> MISNNAPAKMVLNSIM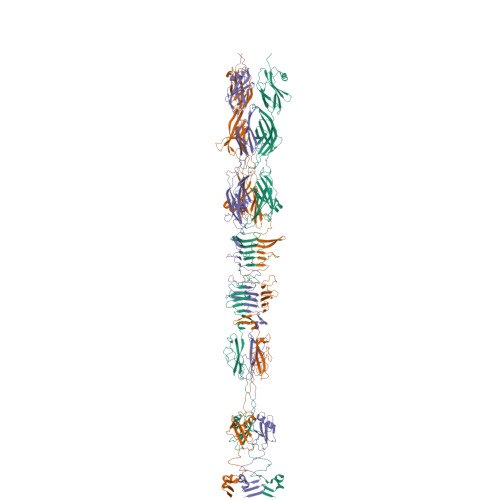TGYTLAYVQHSIYTDYDVIGRSFWLKVEESIDRRDYTGVDTFFVMINNLTPSTSYEIQGAFYDSIIDSELLEAKIGINLSNETNFRTKEKPIIVAARSESEPVDVGVGAPIVVVETTGEASYCTIELKSTASEDSEWVKYYIGALGPTIKFGGVPVGDYKIRISGQVTMPDGVTVDSSGYYEYPSVFTVAYNFVPPTAPTNIAFKAARIADGKERYDARIEWDWERGAGANVREFLVTYINSEEYARTGWAKAQKINVGAARAATIISFPWKVEHTFKVSSIAWGPNRQDITESAPATFILNEDTPLDNSFVNETGIDVNYAFIKGSMKEGEIWKQTFLIDAATGAINIGLLDEEGKAPISFDPINRVVNVDGKVITRDINAANFIMTNLSGEDNPAIYTQGKSWGDNNSGIWMGMDNTSAKAKLDIGNATQWIRYDGDVLRISSGVVIGTPNGDVDLGTGMQGKQTVFVYKLATSLPAKPLEQDYPPPGWSKTPPNRTDMTQNIYATTGTLDPVTNRLLEGTSWSDVVQWSGTEGTIGHDGQRGPGMYSVGIAGLGGWDDGQANSFFTSNFSSAPVKYDVLTEYKSDAPGTAFTRQWNGSGWVNPAMVLHGNMIVNGTITADKIVAGNAFLSQIGVNTIYDRAAALSGNPEAQYKMKIDLVNGYIHIR> SMFNVSNNVAPSRYQGPSSTSVTPNAFHDVPSLGQKVGAGSQKDVFHSRQDPRQCICLFRPGTTGSIPAEQYAQKELETTKQLKNLGFPVVDAHALVKHQG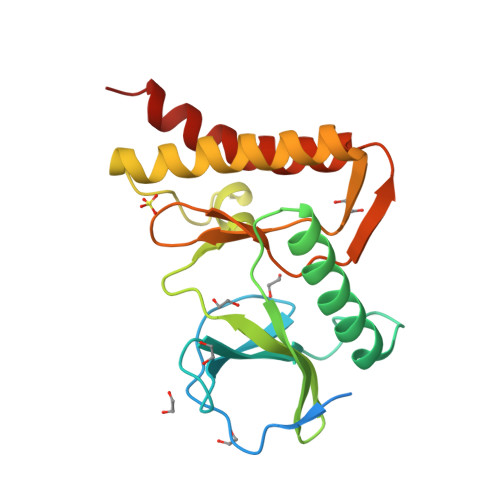SVGVAKDFIHNALDSEDIVNNKKSLPDNLKFNKNVLEDCNAIIRRLKNLEVHIEDLQFLVDHNGHVLINDPRDVVRSSPDKSISKVNELRSHALNNLLDIDSD>MHHHHHHTLGDQGGQGQEPPPEPRITLKVGGQPVTFLVDTGAQHSVLTQNPGPLSDKSAWVQGATGGKRYRWTTDRKVHLATGKVTHSFLHVPDCPYPLLGRDLLTKLKAQIHFEGSGAQVVGPMGQPLQ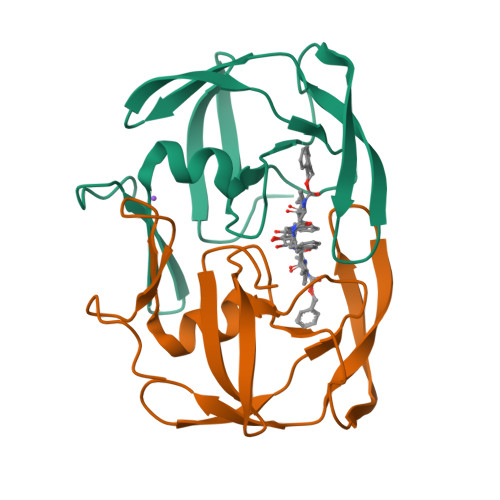VL[2x]>[2x]GHMGSSGGMSSRKRGITPSRDQVRRKKLSIEETDSIEVVCRLCPYTGSTPSLIAIDEGSIQTVLPPAQFRRENAPQVEKVFRFGRVFSENDGQATVFERTSVDLILNLLKGQNSLLFTYGVTGSGKTYTMTGKPTETGTGLLPRTLDVIFNSINNRVEKCIFYPSALNTFEIRATLDAHLKRHQM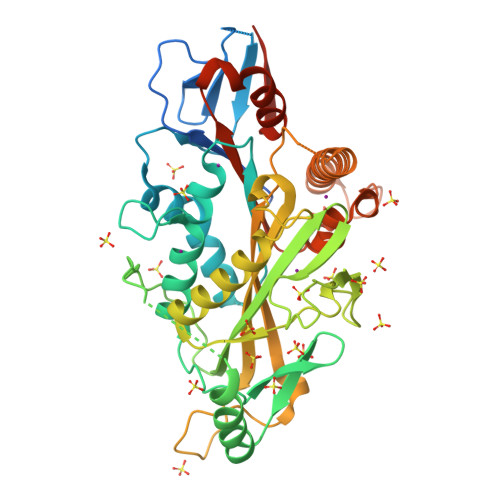AADRLSTSREITDRYCEAIKLSGYNDDMVCSVFVTYVEIYNNYCYDLLEDARNGVLTKREIRHDRQQQMYVDGAKDVEVSSSEEALEVFCLGEERRRVSSTLLNKDSSRSHSVFTIKLVMAPRAYETKSVYPTMDSSQIIVSQLCLVDLAGSERAKRTQNVGERLAEANSINQSLMTLRQCIEVLRRNQKSSSQNLEQVPYRQSKLTHLFKNYLEGNGKIRMVICVNPKPDDYDENMSALAFAEESQTIEVKKQVERMPSERIP> DITVYNGQHKEAATAVAKAFEQETG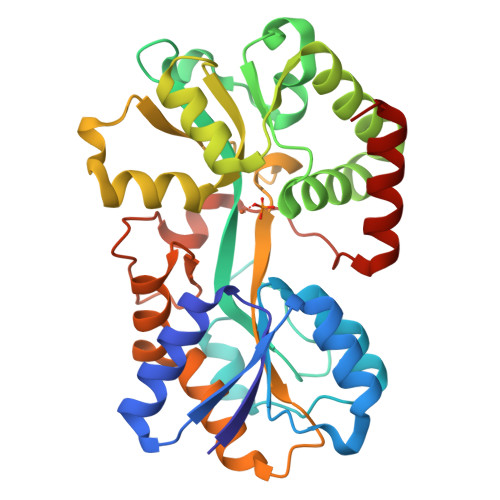IKVTLNSGKSEQLAGQLKEEGDKTPADVFYTEQTATFADLSEAGLLAPISEQTIQQTAQKGVPLAPKKDWIALSGRSRVVVYDHTKLSEKDMEKSVLDYATPKWKGKIGYVSTSGAFLEQVVALSKMKGDKVALNWLKGLKENGKLYAKNSVALQAVENGEVPAALINNYAWYNLAKEKGVENLKSRLYFVRHQDPGALVSYSGAAVLKASKNQAEAQKFVDFLASKKGQEALVAARAEYPLRADVVSPFNLEPYEKLEAPVVSATTAQDKEHAIKLIEEAGLK>[2x]MRG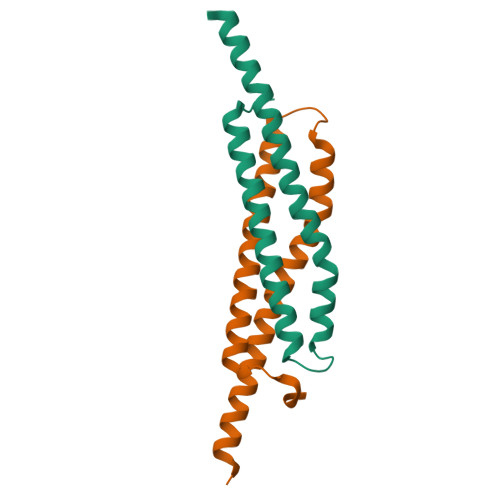SHHHHHHGSMAQIKLTPEELRSSAQKYTAGSQQVTEVLNLLTQEQAVIDENWDGSTFDSFEAQFNELSPKITEFAQLLEDINQQLLKVADIIEQTDADIASQISG> MLDTNMKTQLRAYLEKLTKPVELIATLDDSAKSAEIKELLAEIAELSDKVT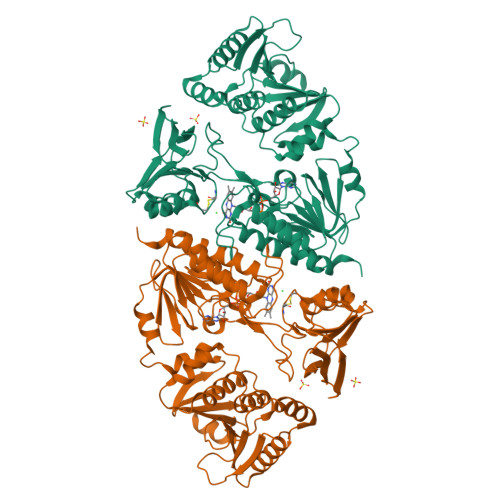FKEDNTLPVRKPSFLITNPGSQQGPRFAGSPLGHEFTSLVLALLWTGGHPSKEAQSLLEQIRDIDGDFEFETYYSLSCHNCPDVVQALNLMAVLNPRIKHTAIDGGTFQNEITERNVMGVPAVFVNGKEFGQGRMTLTEIVAKVDTGAEKRAAEALNKRDAYDVLIVGSGPAGAAAAVYSARKGIRTGLMGERFGGQVLDTVDIENYISVPKTEGQKLAGALKAHVSDYDVDVIDSQSASKLVPAATEGGLHQIETASGAVLKARSIIIATGAKWRNMNVPGEDQYRTKGVTYCPHCDGPLFKGKRVAVIGGGNSGVEAAIDLAGIVEHVTLLEFAPEMKADQVLQDKVRSLKNVDIILNAQTTEVKGDGSKVVGLEYRDRVSGDIHSVALAGIFVQIGLLPNTHWLEGALERNRMGEIIIDAKCETSVKGVFAAGDCTTVPYKQIIIATGEGAKASLSAFDYLIRTKIA Adenosine undergoes ATP-dependent phosphorylation catalyzed by adenosine kinase (ADK). In plants, ADK also phosphorylates cytokinin ribosides, transport forms of the hormone. We discovered that maize and moss enzymes can form dimers upon increasing protein concentration, setting them apart from the monomeric human and protozoal ADKs. Structural and kinetic analyses revealed a catalytically inactive unique dimer.

Since the ATP site was accessible, we obtained a complex of ZmADK2 with AMP-PCP in the open conformation. The Ado moiety of ATP is surrounded by hydrophobic residues. Indeed, its ring is located between Ile328 and Ala295 on one side, and Ala265 with Gly264 on the other, forming multiple hydrophobic contacts. The O2' atom of the ribose moiety is bound directly to the SG atom of Cys321, and the O3' atom is H-bonded via a water molecule to the main chain oxygen atom of Gly264 and the nitrogen of Gln263. The α-phosphate group forms a hydrogen bond with the OG1 atom of Thr262. The β-phosphate group is H-bonded to Asn220, and both the β- and γ-phosphate groups interact with Glu223 via two water molecules. Finally, the negatively charged γ-phosphate moiety establishes an electrostatic interaction with the positively charged side chain of Arg130. AP5A in ZmADK3 and AMP-PCP in ZmADK2 adopt the same conformation and position in the ATP-binding site.

>[2x]MGSSHHHHHHSQDPNSSSMAASEGVLLGMGNPLLDISAVVDDAFLTKYDIKLNNAILAEEKHLPMYDELASKSNVEYIAGGATQNSIRVAQWMLQTPGATSYMGCIGKDKFGEEMKKNAQAAGVTAHYYEDETAPTGTCAVCVVGGERSLIANLSAANCYKSEHLKRPENWALVEKAKYIYIAGFFLTVSPDSIQLVAEHAAANNKVFLMNLSAPFICEFFRDAQEKVLPYADYIFGNETEAKIFAKVRGWETENIEEIALKISQLPLASGKQKRIAVITQGADPVVVAEDGKVKTFPVILLPKEKLVDTNGAGDAFVGGFLSQLVLGKGIEDCVRAGCYAANVIIQRPGCTYPEKPDFN>SMHPLTDASANDALHAYDTAVKLAFDRIVPVLKRLSALQHEDDFVGRAQAIALEELGFPLPEPILDTAWVSQLDMRTLYAWCVFETYEQTSEAFFRDDPLQGQPGSPSAEAFDRFLLDCGFHLLDITPCADGRLAHAIGFGLRLPFSSVRRRPHAGALFDVENTVNRWVKTEHRRYREAQPNPAHADTRYLKVALYHFSSLDPQHEGCAAHGSDDALAASCGLSRLKDFQQAVENSFCCGASVDLLLMGIDTDTDAIRVHVPGMDGSTRLDRWLDARDVYDATLGLPPDQARQRVSALVQEAAASVPDPGMVTLVARLFEHNISQIDYVRQFHGGAYDDAGHAERFIGVGIGFKEIHLRNLTYFAYMDTVEEGAADLDVGVKIFKGLNVSRGLPVPVVVRFDYHGQVPGARDRAVRHCQRVQTAIESRYPELFQQGLLHALLTVRDQDRHTPAEAVGSTIVF[6x]

Proteinaceous microcompartments, called carboxysomes, play a critical role in CCM function, housing two enzymes to enhance CO2 fixation: carbonic anhydrase (CA) and Rubisco. Here, the CA converts HCO3− to CO2 to elevate luminal CO2, promoting Rubisco-catalyzed CO2 reduction. Correspondingly, microbial and biochemical studies have established an absolute requirement for CA activity within the carboxysome The α-carboxysome contains a highly divergent β-CA known as CsoSCA, characterization of which has occurred exclusively through the isoform from the chemoautotroph Halothiobacillus neapolitanus. Our results show that the Cyanobium CsoSCA is allosterically activated by the Rubisco substrate ribulose-1,5-bisphosphate and forms a hexameric trimer of dimers.

To understand the structural basis for RuBP activation, CsoSCA was co-crystallized with RuBP. Diffracting crystals were obtained almost exclusively in saturating levels of RuBP with the final CsoSCA crystal structure solved through molecular replacement to a resolution of 2.3 Å. The resulting structure showed a homohexameric trimer of dimers consistently arranged in the asymmetric unit with P212121 symmetry. A metal ion is evident at each apex, coordinated by a His3(H2O)3 octahedral coordination sphere, comprising His155 donated by a distinct monomer. The electron density and coordination geometry are consistent with a zinc ion. Density corresponding to a HCO3− ion was observed at one of the trimer apices. While variations in omit map density at these positions were observed, given the consistency of this density across each chain, the dependence on RuBP for crystallization, and the observation that RuBP was an allosteric activator of CA, we were confident in the modeling of RuBP at this site. Most notably, RuBP curls around Lys469, mediating multiple H-bonds with the ligand. The Cys2His(H2O) tetrahedral coordination of the catalytic zinc ion typical of β-CAs is maintained, and the overarching active site is highly homologous between each CsoSCA isoform. Manual inspection of H-bonds within the protein identified a network linking the catalytic Asp246 backbone and the Arg266 side chain that, in turn, binds RuBP, mediated by a water molecule and Leu249 backbone groups.> MASGGSGGVSVPALWSEVNRYGQNGDFTRALKTVNKILQINKDDVTALHCKVVCLIQNGSFKEALNVINTHTKVLANNSLSFEKAYCEYRLNRIENALKTIESANQQTDKLKELYGQVLYRLERYDECLAVYRDL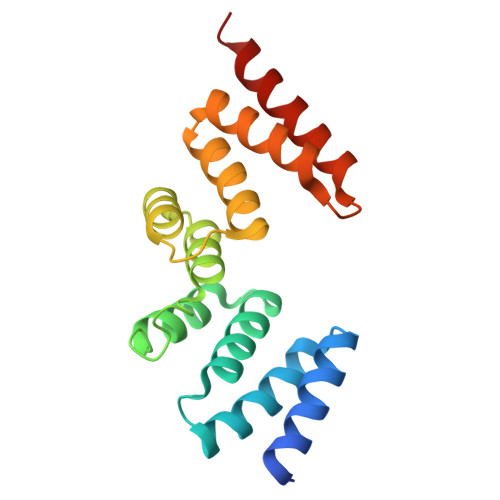VRNSQDDYDEERKTNLSAVVAAQSNWEK>[6x]MTSAEMTSPNNNSEHQAIAKMRTMIEGFDDISHGGLPIGRSTLVSGTSGTGKTLFSIQFLYNGIIEF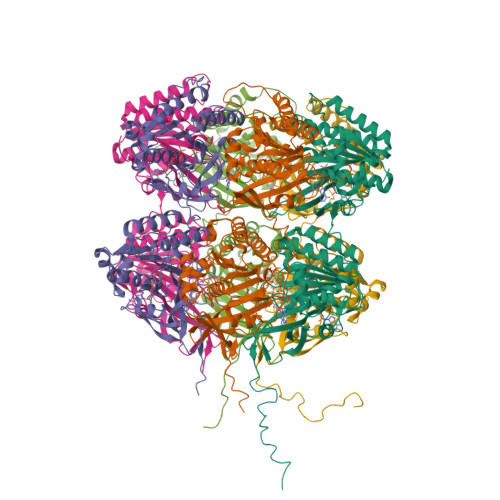DEPGVFVTFEETPQDIIKNARSFGWDLAKLVDEGKLFILDASPDPEGQEVVGGFDLSALIERINYAIQKYRARRVSIDSVTSVFQQYDASSVVRRELFRLVARLKQIGATTVMTTERIEEYGPIARYGVEEFVSDNVVILRNVLEGERRRRTLEILKLRGTSHMKGEYPFTITDHGINIFPLGAMRLTQRSSNVRVSSGVVRLDEMCGGGFFKDSIILATGATGTGKTLLVSRFVENACANKERAILFAYEESRAQLLRNAYSWGMDFEEMERQNLLKIVCAYPESAGLEDHLQIIKSEINDFKPARIAIDSLSALARGVSNNAFRQFVIGVTGYAKQEEITGLFTNTSDQFMGAHSITDSHISTITDTIILLQYVEIRGEMSRAINVFKMRGSWHDKAIREFMISDKGPDIKDSFRNFERIISGSPTRITVDEKSELSRIVRGVQEKGPES The Type VI-D CRISPR-Cas system employs an RNA-guided RNase Cas13d with minimal targeting constraints to combat viral infections. The Ruminococcus sp. WYL1 (RspWYL1) has been demonstrated to significantly boost Cas13d’s target selectivity and RNase activity (both the cis- and trans-cleavage). Through structural and biophysical approaches, we reveal that the full-length RspWYL1 possesses a novel three-domain architecture and preferentially binds ssRNA with high affinity. Specifically, the N-terminus of RspWYL1 harbors a ribbon-helix-helix motif reminiscent of transcriptional regulators; the central WYL domain of RspWYL1 displays a Sm-like β-barrel fold; and the C-terminal domain of RspWYL1 primarily contributes to the dimerization of RspWYL1 and may regulate the RspWYL1 function via a large conformational change.

To gain mechanistic insights into the modulatory role of WYL1 in the newly discovered Type VI-D CRISPR-Cas system, we determined the crystal structure of the full-length WYL1 protein from Ruminococcus sp. (RspWYL1) by the single-wavelength anomalous dispersion (SAD) method. Each asymmetric unit in the crystal structure contains two RspWYL1 molecules, forming a diamond-shaped, ∼95 × 85 × 80 Å homodimer. The RspWYL1 protomer comprises three domains, which are arranged in a triangular fashion. The two protomers in the RspWYL1 dimer spatially arrange side-by-side, and interact with each other mainly through their NTD and CTD domains. On the other hand, the CTD−CTD interactions involve 16 residues to generate an interface area of ∼1300 Å2, accounting for the majority of intermolecular interactions of the RspWYL1 homodimer (∼60%). The NTD of RspWYL1 harbors two RHH motifs, denoted RHH1 and RHH2. However, the two RHH motifs of RspWYL1 are in a single polypeptide chain and fold together in a pseudo-2-fold symmetry, highlighting the diversity of the RHH superfamily. Instead, an unexpected charged residue (Arg133) is present at the position 4 that would cause steric clashes with the major groove of dsDNA, implying that RspWYL1 might disfavor dsDNA. Our structural analysis revealed that the WYL domain projects out from the dimerization interface of the RspWYL1 homodimer, and adopts a Sm-like β-barrel structure. Within the RspWYL1 homodimer, the relative orientations of the two CTDs differ significantly.

>[2x]GMLIPPSTFLPKRDKNVPYIAEVQSIPLSPSAYSVIIKDKSIFETSLSPNGSVSMSSFLTSIFDSAYIASLKYKSDDNYKYIGIPLLNAFVEWQIEEIDDSLDDKSKEIIKSYLISKLSAKYEKTKTENAVRVRLSICRDLYDTLSSDDLYYENKVYSLTLRRFLKAVYEDYALLSDCERERLIFADNIIKINEVIKQNGSRYYSFIYAYSNMYSREKRRIRLIPYRIVSDEYKMYNYLVCLSDEKSAGKEFKADSYRISRLSGLSIAEKLSQKEYSSVTEYERLKEGHVKSVKHLLSDPRFGSDESDISKVYLTEKGVEMFRKILYQRPILKGNEKPKPNTVNEFISPPIQVKYYFNKFGKDGVILSPSDSFEEMRTLYVEGADAYNREVEM> MAAAAPPPPPTAAPEPNMVAPLISPIGHPMFSRIRLATPSDVPFIHKLIHQMAVFERLTHLFSATESGLASTLFTSRPFQSFTVFLLEV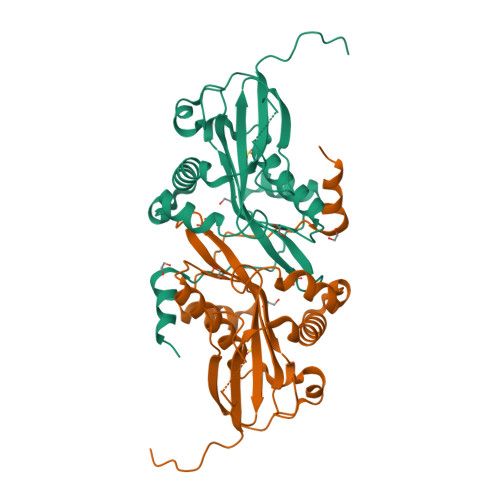SRSPFPATITSSPSPDFTPFFKTHNLDLPIDDPESYNFSPDMLNDVVVAGFVLFFPNYSSFLSKPGFYIEDIFVREPYRRKGFGSMLLTAVAKQAVKMGYGRVEWVVLDWNVNAIKFYEQMGAQILQEWRVCRLTGDALEAFDQVNI>MLNAWHLPVPPFVKQSK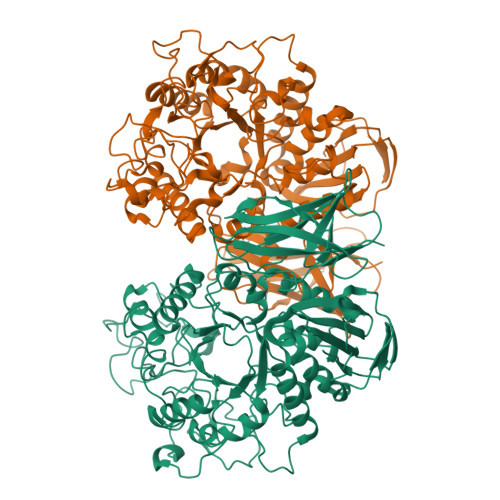DQLLITLWLTGEDPPQRIMLRTEHDNEEMSVPMHKQRSQPQPGVTAWRAAIDLSSGQPRRRYSFKLLWHDRQRWFTPQGFSRMPPARLEQFAVDVPDIGPQWAADQIFYQIFPDRFARSLPREAEQDHVYYHHAAGQEIILRDWDEPVTAQAGGSTFYGGDLDGISEKLPYLKKLGVTALYLNPVFKAPSVHKYDTEDYRHVDPQFGGDGALLRLRHNTQQLGMRLVLDGVFNHSGDSHAWFDRHNRGTGGACHNPESPWRDWYSFSDDGTALDWLGYASLPKLDYQSESLVNEIYRGEDSIVRHWLKAPWNMDGWRLDVVHMLGEAGGARNNMQHVAGITEAAKETQPEAYIVGEHFGDARQWLQADVEDAAMNYRGFTFPLWGFLANTDISYDPQQIDAQTCMAWMDNYRAGLSHQQQLRMFNQLDSHDTARFKTLLGRDIARLPLAVVWLFTWPGVPCIYYGDEVGLDGKNDPFCRKPFPWQVEKQDTALFALYQRMIALRKKSQALRHGGCQVLYAEDNVVVFVRVLNQQRVLVAINRGEACEVVLPASPFLNAVQWQCKEGHGQLTDGILALPAISATVWMNAAALEHHHHHH[2x]>[2x]MAQTDTYPNIEAL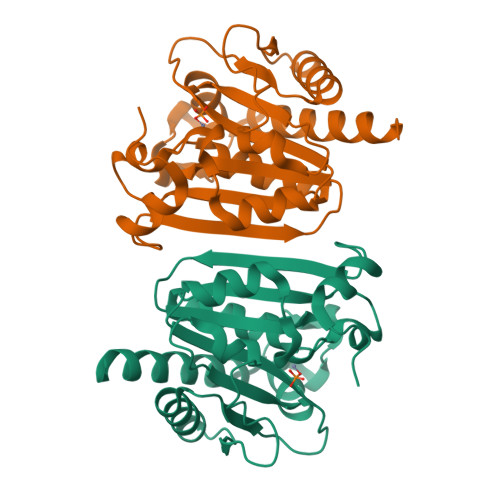ENAETVGVAYNIEVKRQNPSMIYFSPHAGGIEVGTTELIYRVVELTGGSLYLFQGLLPSGNSRLHVTSTHFDEPMAVCMLSKHTDAVSFHGYKDDYNKNTLVGGLNTELRNLIVSKLNSKGIAAEVATDRFTATDPDNIVNRCASGKGVQLEISSAQRRAFFQNNDWSKANRGNVTQEFLDYAEAIKEAEAEYYGLEHHHHHH> KESALR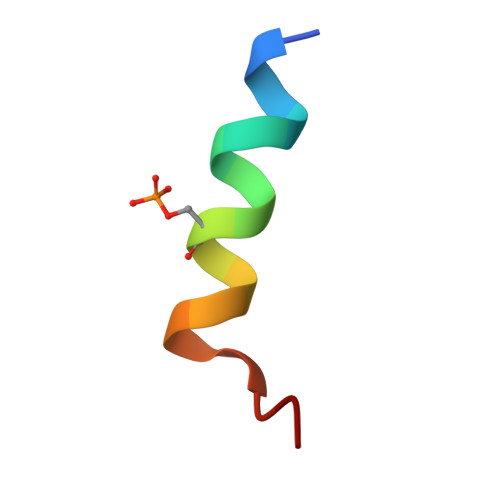KQSLYLKFDPLL>GLTPEQKQKKAALSASEGEEVPQDKAPSHVPFLLIGGGTAAFAAARSIRARDPGARVLIVSEDPELPYMRPPLSKELWFSDDPNVTKTLRFKQWNGKERSIYFQPPSFYVSAQDLPHIENGGVAVLTGKKVVQLDVRDNMVKLNDGSQITYEKCLIATGSTPRSLSAIDRAGAEVKSRTTLFRKIGDFRSLEKIS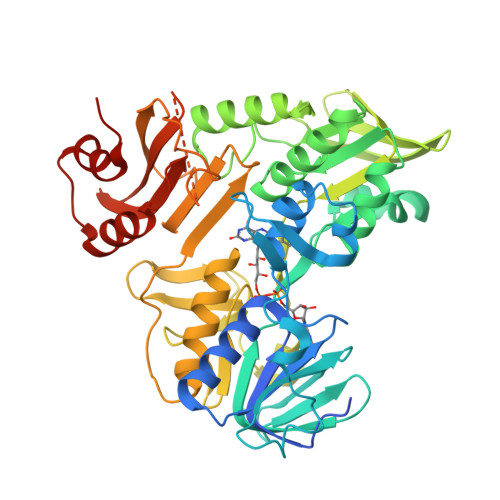REVKSITIIGGGFLGSELACALGRKARALGTEVIQLFPEKGNMGKILPEYLSNWTMEKVRREGVKVMPNAIVQSVGVSSGKLLIKLKDGRKVETDHIVAAVGLEPNVELAKTGGLEIDSDFGGFRVNAELQARSNIWVAGDAACFYDIKLGRRRVEHHDHAVVSGRLAGENMTGAAKPYWHQSMFWSDLGPDVGYEAIGLVDSSLPTVGVFAKATAQDNPKSATEQSGTGIRSESETESEASEITIPPSTPAVPQAPVQGEDYGKGVIFYLRDKVVVGIVLWNIFNRMPIARKIIKDGEQHEDLNEVAKLFNIHEDLVPR[2x]> GSSGSSGYQPTYNPTLPYKRPIPGGLSVGMSVYIQGMAKENMRRFHVNFAVGQDDGADVAFHFNPRFDGWDKVVFNTMQSGQWGKEE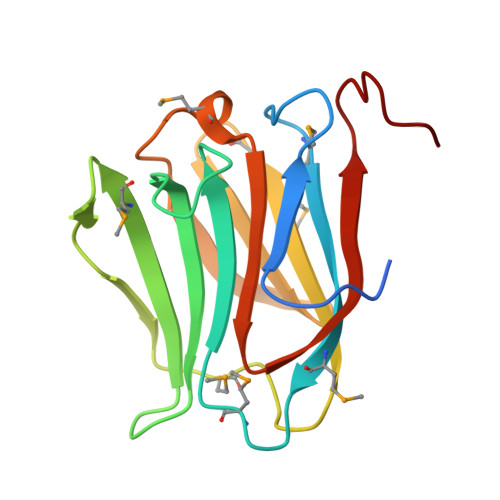KKKSMPFQKGKHFELVFMVMPEHYKVVVNGNSFYEYGHRLPVQMVTHLQVDGDLELQSINFLGGQPAAAPY>[4x]SFGRDACSEMSIDGLCQCAPIMSEYEIICPANAENPTFRLTIQPKDYVQIMCNLTDTTDYQQLPKKLRIGEVDRVQMRRCMLPGHTPIASILDYLGIVSPTTLIFESDNLGMNITRQHLDRLHGLKRFRFTTRRLTHIPANLLTDMRNLSHLELRANIEEMPSHLFDDLENLESIEFGSNKLRQMPRGIFGKMPKLKQLNLASNQLKSVPDGIFDRLTSLQKIWLHTNPWDCSCPRIDYLSRWLNKNSQKEQGSAKCSGSGKPVRSIICPTTGENLYFQ

endogenous protein Spätzle (Spz) that is unique to insects. related to mammalian growth factors, such as the nerve growth factor (NGF) (Hoffmann et al., 2008; Mizuguchi et al., 1998). segregated in two blocks capped by cysteine-rich regions. dimerization followed by receptor clustering with cell-specific signaling molecules.

in truncating the receptor following the hybrid LRR technology (Kim et al., 2007). technology and referred to as TollN6-VLR (Kim et al., 2007). arc-shape typical of the leucine-rich repeat (LRR) fold. is tethered to the first beta-strand by a disulfide bond (Cys34-Cys45). disulfide bonds stabilize the LRRNT cap in Toll. anchors the fourth strand of the cap to the first leucine-rich repeat (LRR1). five-residue-long beta-strands in LRR1–4 and three-residue-long in LRR5 and LRR6. in the first block of LRRs in Toll to form a hydrophobic spine. C-terminal capping structure (LRRCT) of VLR B.61. to protect the hydrophobic core of the last LRR from solvent exposure.> ASRSQAEDVRVEGSFPVTMLPGDGVGPELMHAVKEVFKAAAVPVEFQEHHLSEVQNMASEEKLEQVLSSMKENKVAIIGKIHTPMEYKGELASYDMRLRRKLDLFANVVHVKSLPGYMTRHNNLDLVIIREQTEGEYSSLEHESARGVIECLKIVTR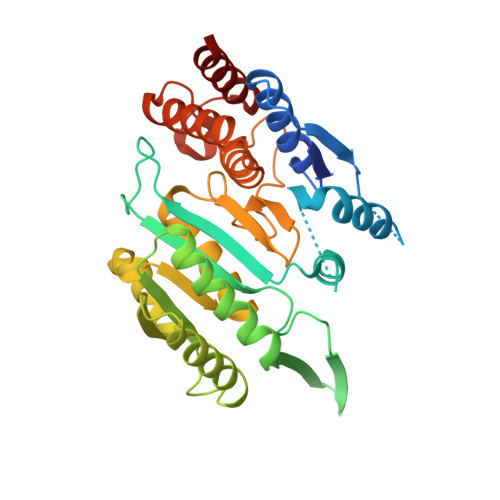AKSQRIAKFAFDYATKKGRGKVTAVHKANIMKLGDGLFLQCCEEVAELYPKIKFETMIIDNCCMQLVQNPYQFDVLVMPNLYGNIIDNLAAGLVGGAGVVPGESYSAEYAVFETGARHPFAQAVGRNIANPTAMLLSASNMLRHLNLEYHSSMIADAVKKVIKVGKVRTSDMGGYATCHDFTEEICRRVKDLDENLYFQ N-{1-[(2-aminoethyl)sulfonyl]piperidin-4-yl}-5-cyclopropyl-1,2-oxazole-3-carboxamide | C14 H22 N4 O4 S | 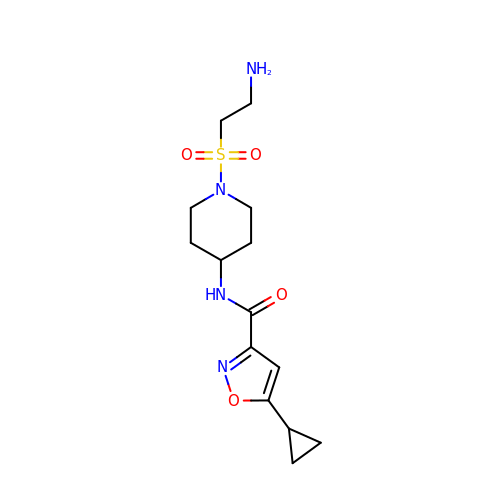AMCHZZBLDUVCGF-UHFFFAOYSA-N1,3-dithiolane-2-carboxylic 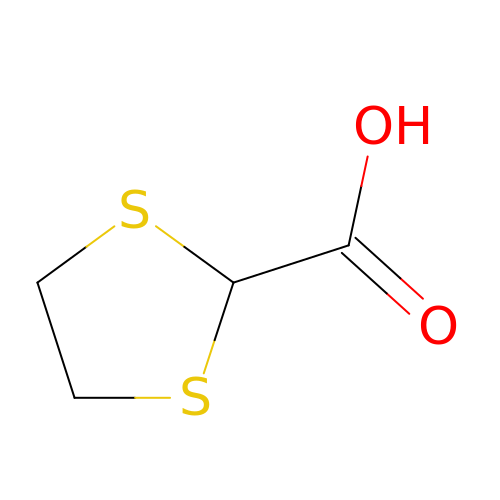acid | C4 H6 O2 S2 | DSOVOUOPKYLGID-UHFFFAOYSA-N>LPNITILATGGTIAGGGDSATKSNYTVGKVGVENLVNAVPQLKDIANVKGEQVVNIGSQDMNDNVWLTLAKKINTDCDKTDGFVITHGTDTMEETAYFLDLTVKCDKPVVMVGAMRPSTSMSADGPFNLYNAVVTAADKASANRGVLVVMNDTVLDGRDVTKTNTTDVATFKSVNYGPLGYIHNGKIDYQRTPARKHTSDTPFDVSKLNELPKVGIVYNYANASDLPAKALVDAGYDGIVSAGVGNGNLYKSVFDTLATAAKTGTAVVRSSRVPTGATTQDAEVDDAKYGFVASGTLNPQKARVLLQLALTQTKDPQQIQ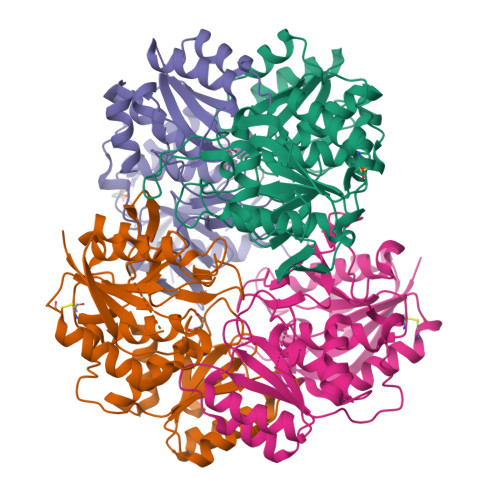QIFNQY[4x]> MLEADDQGCIEEQGVEDSANEDSVDAKPDRSSFVPSLFSKKKKNVTMRSIKTTRDRVPTYQYNMNFEKLGKCIIINNKNFDKVTGMGVRNGTDKDAEALFKCFRSLGFDVIVYND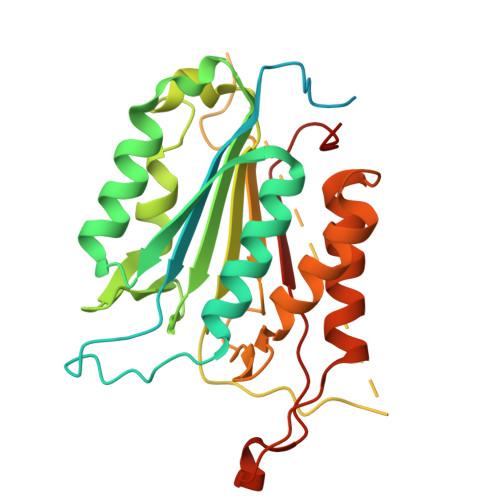CSCAKMQDLLKKASEEDHTNAACFACILLSHGEENVIYGKDGVTPIKDLTAHFRGDRSKTLLEKPKLFFIQACRGTELDDGIQADSGPINDTDANPRYKIPVEADFLFAYSTVPGYYSWRSPGRGSWFVQALCSILEEHGKDLEIMQILTRVNDRVARHFESQSDDPHFHEKKQIPCVVSMLTKELYFSQ>QLLFNKTKSVEFTFGNDTVVIPCFVTNMEAQNTTEVYVKWKFKGRDIYTFDGALNKSTVPTDFSSAKIEVSQLLKGDASLKMDKSDAVSHTGNYTCEVTEL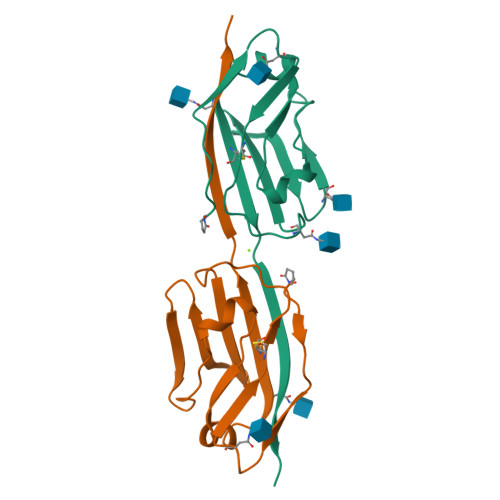TREGETIIELKYRVVSWSTRHHHHHH[4x]>[2x]SMREYEHVRRDLDPNEVWEIVGELGDGAFGKVYKAKNKETGALAAAKVIETKSEEELEDYIVEIEILATCDHPYIVKLLGAYYHDGKLWIMIEFCPGGAVDAIMLELDRGLTEPQIQVVCRQMLEALNFLHSKRIIHRDLKAGNVLMTLEG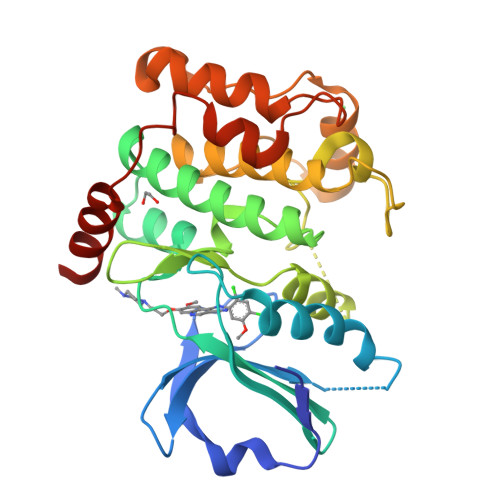DIRLADFGVSAKNLKTLQKRDSFIGTPYWMAPEVVMCETMKDTPYDYKADIWSLGITLIEMAQIEPPHHELNPMRVLLKIAKSDPPTLLTPSKWSVEFRDFLKIALDKNPETRPSAAQLLEHPFVSSITSNKALRELVAEAKAE> HMDPDELPLDEHCERLPYDASKWEFPRDRLNLGKPLGRGAFGQVIEADAFGIDKTATCRTVAVKMLKEGATHSEHRALMSELKILIHIGHHLNVVNLLGACTKPGGPLMVIVEFCKFGNLSTYLRSKRNEFVPYKTPEDLYKDFLTLEHLICYSFQVAKGMEFLASRKCIHRDLAARNILLSEKNVVKICDFGLARDIYKDPDYVRKGDARLPLKWMAPETIFDRVYTIQSDVWSFGVLLWEIF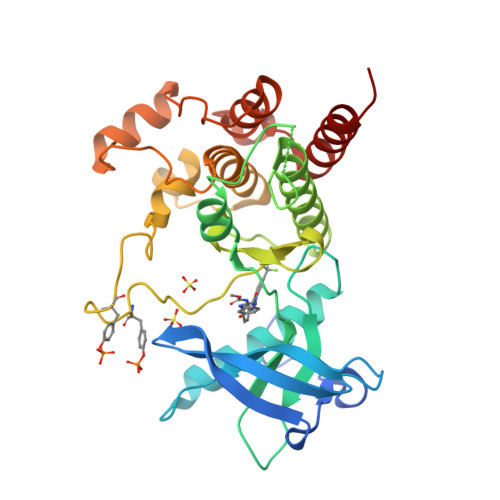SLGASPYPGVKIDEEFCRRLKEGTRMRAPDYTTPEMYQTMLDCWHGEPSQRPTFSELVEHLGNLLQANAQQD>[2x]CSLIPDYQRPEAPVAAAYPQGQAYGQNTGAAAVPAADIGWREFFRDPQLQQLIGVALEN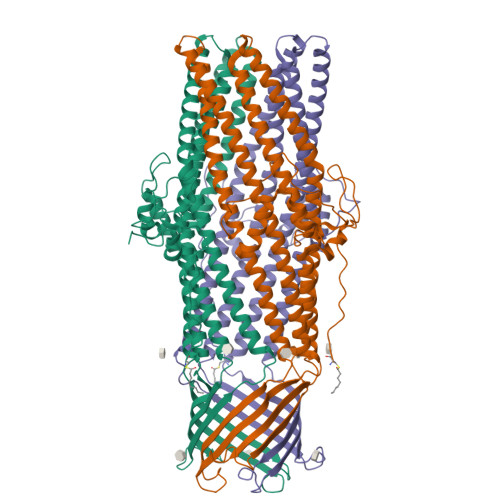NRDLRVAALNVEAFRAQYRIQRADLFPRIGVDGSGTRQRLPGDLSTTGSPAISSQYGVTLGTTAWELDLFGRLRSLRDQALEQYLATEQAQRSAQTTLVASVATAYLTLKADQAQLQLTKDTLGTYQKSFDLTQRSYDVGVASALDLRQAQTAVEGARATLAQYTRLVAQDQNALVLLLGSGIPANLPQGLGLDQTLLTEVPAGLPSDLLQRRPDILEAEHQLMAANASIGAARAAFFPSISLTANAGTMSRQLSGLFDAGSGSWLFQPSINLPIFTAGSLRASLDYAKIQKDINVAQYEKAIQTAFQEVADGLAARGTFTEQLQAQRDLVKASDEYYQLADKLFRTGVDNYGTLLAAQASLFTAQQQLITDRLNQLTSEVNLYKALGGGWNQQTVTQQQTAKKEDPQAHHHHHH>[2x]MAMKISVSKNDLENALRYLQAFLDKKDASSIASHIHLEVIKEKLFLKASDSDIGLKSYIFTQSSDKEGVGTINGKKFLDIISCLKDSNIILETKDDSLAIKQNKSSFKLPMFDADEFPEFPVI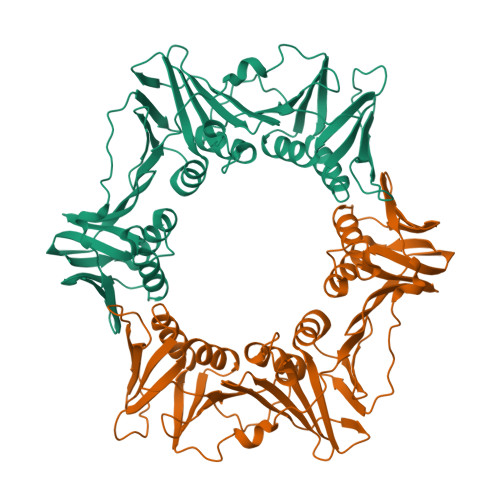DPKVSIEVNAPFLVDAFKKIAPVIEQTSHKRELAGILMQFDQKHQTLSVVGTDTKRLSYTQLEKISIHSTEEDISCILPKRALLEILKLFYENFSFKSDGMLAVIENEMHTFFTKLIDGNYPDYQKILPKEYISSFTLGKEEFKESIKLCSSLSSTIKLTLEKNNALFESLDSEHSETAKTSVEIEKGLDIEKAFHLGVNAKFFLEALNALGTTQFVLRCNEPSSPFLIQESLDEKQSHLNAKISTLMMPITLELHHHHHH>MGSSHHHHHHSSGLENLYFQGSDQVQKVDQYLYHMRLSDETLLEISKRFRKEMEKGLGATTHPTAAVKMLPTFVRSTPDGTEHGEFLALDLGGTNFRVLWVKVTDNGLQKVEMENQIYAIPEDIMRGSGTQLFDHIAECLANFMDKLQIKDKKLPLGFTFSFPCHQTKLDESFLVSWTKGFKSSGVEGRDVVALIRKAIQRRGDFDIDIVAVVNDTVGTMMTCGYDDHNCEIGLIVGTGSNACYMEEMRHIDMVEGDEGRMCINMEWGAFGDDGSLNDIRTEFDQEIDMGSLNPGKQLFEKMISGMYMGELVRLILVKMAKEELLFGGKLSPELLNTGRFETKDISDIEGEKDGIRKAREVLMRLGLDPTQEDCVATHRICQIVSTRSASLCAATLAAVLQRIKENKGEERLRSTIGVDGSVYKKHPHFAKRLHKTVRRLVPGCDVRFLRSEDGSGKGAAMVTAVAYRLADQHRARQKTLEHLQLSHDQLLEVKRRMKVEMERGLSKETHASAPVKMLPTYVCATPDGTEKGDFLALDLGGTNFRVLLVRVRNGKWGGVEMHNKIYAIPQEVMHGTGDELFDHIVQCIADFLEYMGMKGVSLPLGFTFSFPCQQNSLDESILLKWTKGFKASGCEGEDVVTLLKEAIHRREEFDLDVVAVVNDTVGTMMTCGFEDPHCEVGLIVGTGSNACYMEEMRNVELVEGEEGRMCVNMEWGAFGDNGCLDDFRTEFDVAVDELSLNPGKQRFEKMISGMYLGEIVRNILIDFTKRGLLFRGRISERLKTRGIFETKFLSQIESDCLALLQVRAILQHLGLESTCDDSIIVKEVCTVVARRAAQLCGAGMAAVVDRIRENRGLDALKVTVGVDGTLY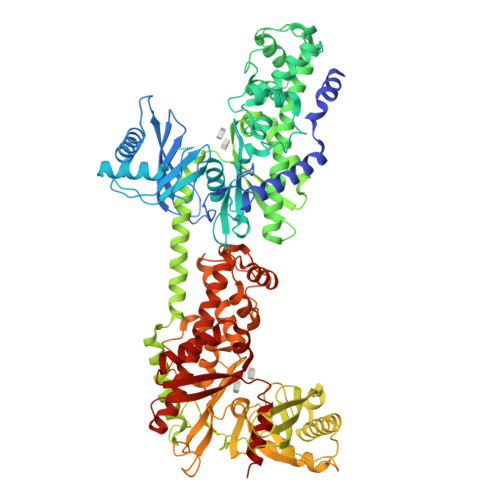KLHPHFAKVMHETVKDLAPKCDVSFLQSEDGSGKGAALITAVACRIREAGQR[2x]> MF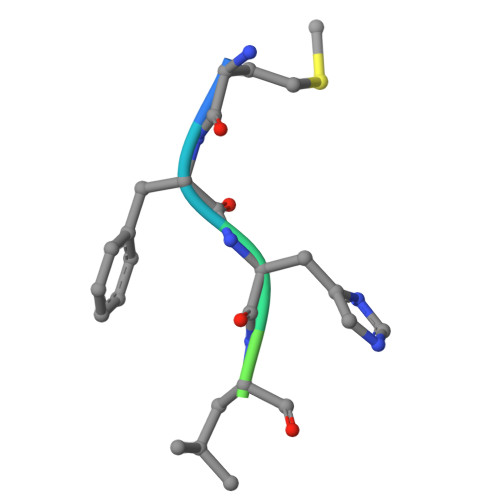HLVGSRRR> GSGAMAQNLDSMLHGTGMKSDSDQKKSENGVTLAPEDTLPFLKCYCSGHCPDDAINNTCITNGHCFAIIEEDDQGETTLASGCMKYEGSDFQCRDTPIPHQRRSIECCRTNLCNQYLQPTLPPVVIGPFF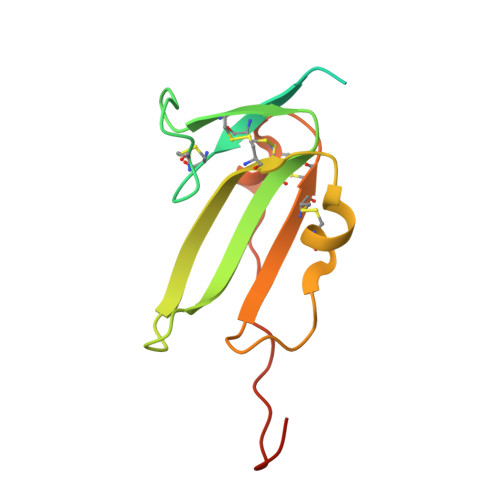DGSIR> MGEQPIFSTRAHVFQIDPNTKKNWVPTSKHAVTVSYFYDSTRNVYRIISLDGSKAIINSTITPNMTFTKTSQKFGQWADSRANTVYGLGFSSEHHLS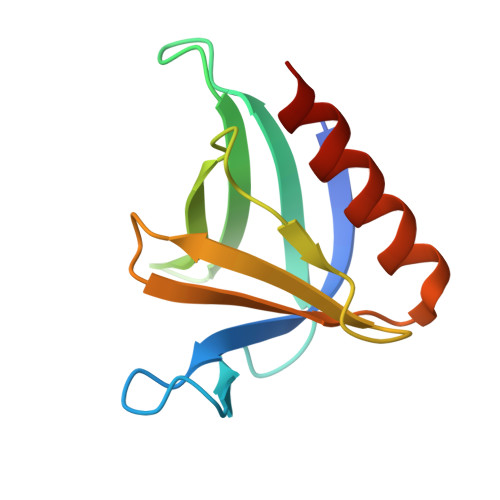KFAEKFQEFKEAAR> SNAMNLKDLLAHRENLMDSAKRARSAITDDMDPADAAQAVENVKSIISEIESTDEAIAARRGV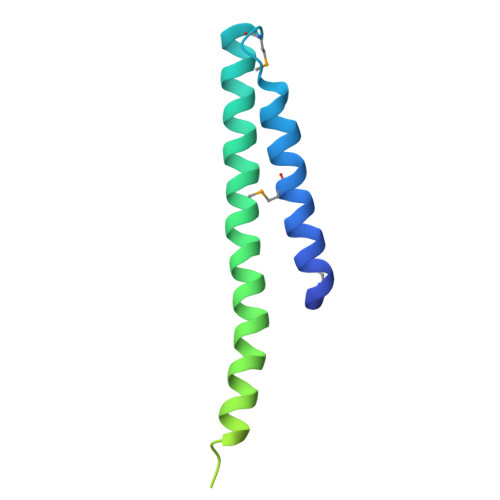SDVTQKLKGLTITERGTENDSAASRSLGEHFVKAAGDRLKNQAAGAHIEYSVPEYQVKEDAHSSPKDLVEGWGTFYQR> AMGSRKSKAELQSEERKRIDELIESGKEEGMKIDLIDGKGRGVIATKQFSRGDFVVEYHGDLIEITDAKKREALYAQDPSTGCY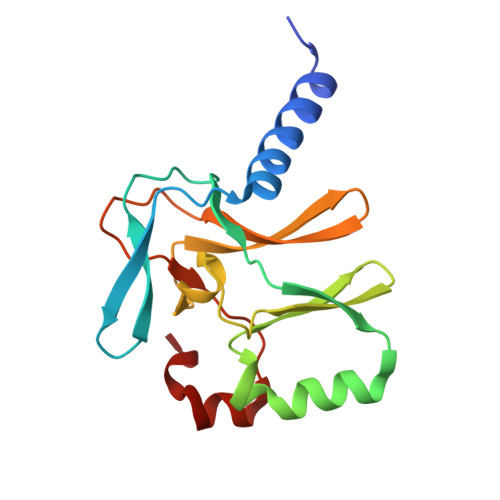MYYFQYLSKTYCVDATRETNRLGRLINHSKSGNCQTKLHDIDGVPHLILIASRDIAAGEELLYDYGDRSKASIEAHPWLKH TRPV6, a representative of the vanilloid subfamily of transient receptor potential (TRP) channels, is the principal calcium uptake channel that captures diet-delivered calcium ions in the gut4–6. TRPV6 is a constitutively open channel. TRPV6 is assembled of four subunits and contains a transmembrane domain (TMD) with the central ion channel pore and an intracellular skirt that is mostly built of ankyrin repeat domains connected to each other by three-stranded β-sheets, N-terminal helices, and C-terminal hooks. The TMD is composed of six transmembrane helices S1–S6 and a re-entrant pore loop (P-loop) between S5 and S6.

Cryo-EM micrographs for hTRPV6-CtD reconstituted in cNW30 nanodiscs in the presence of 114 µM THCV showed evenly dispersed particles with diverse angular coverage. The three-dimensional reconstruction of TRPV6THCV with four-fold rotational symmetry (C4) resulted in a cryo-EM map with the overall resolution of 2.79 Å. High-quality reconstruction of TRPV6THCV identifies three such densities per subunit as representing cholesteryl hemisuccinate (CHS), which was added during protein purification. The first one of the two corresponding THCV binding sites is formed by S5 and S6 of one subunit and S6 of the neighboring subunit and located in the portal connecting the pore and the membrane surrounding TMD. The second site is located next to the first one but it is more peripheral with respect to the pore, surrounded by lipids, including CHS molecules at the vanilloid site (at the interface of S5 and S6 of one subunit and S4 of the neighboring subunit) and at the interface of P-loop of one subunit and S6 of the neighboring subunit. Correspondingly, site 2 is unlikely to cause strong conformational changes in the protein and we propose that site 1 is the main inhibitory site of THCV. In contrast to the apo-state structures of hTRPV6, which have an open conducting pore, the pore in TRPV6THCV is in a fully closed conformation, hydrophobically sealed by the side chains of residues L574 and M578. According to the MD data, the only specific interaction that can stabilize the forward orientation of THCV is the hydrogen bond between the hydroxyl group of THCV and the carbonyl oxygen of L490. The rotation introduces a π-to-α transition in S6, making it entirely α-helical, causes a ~2 helical-turn shortening of S6, a ~2 helical-turn elongation of the TRP helix and repositions M578 so that its side chain points towards the channel pore center. In this position, M578 side chains hydrophobically seal the pore for water and ion conductance, finalizing the open-to-closed state transition. THCV therefore acts as a cog that inserts itself in a cogwheel mechanism of TRPV6 channel and ensures its transition from the open to closed state.

>[4x]MGLSLPKEKGLILCLWSKFCRWFQRRESWAQSRDEQNLLQQKRIWESPLLLAAKDNDVQALNKLLKYEDCKVHQRGAMGETALHIAALYDNLEAAMVLMEAAPELVFEPMTSELYEGQTALHIAVVNQNMNLVRALLARRASVSARATGTAFRRSPCNLIYFGEHPLSFAACVNSEEIVRLLIEHGADIRAQDSLGNTVLHILILQPNKTFACQMYNLLLSYDRHGDHLQPLDLVPNHQGLTPFKLAGVEGNTVMFQHLMQKRKHTQWTYGPLTSTLYDLTEIDSSGDEQSLLELIITTKKREARQILDQTPVKELVSLKWKRYGRPYFCMLGAIYLLYIICFTMCCIYRPLKPRTNNRTSPRDNTLLQQKLLQEAYMTPKDDIRLVGELVTVIGAIIILLVEVPDIFRMGVTRFFGQTILGGPFHVLIITYAFMVLVTMVMRLISASGEVVPMSFALVLGWCNVMYFARGFQMLGPFTIMIQKMIFGDLMRFCWLMAVVILGFASAFYIIFQTEDPEELGHFYDYPMALFSTFELFLTIIDGPANYNVDLPFMYSITYAAFAIIATLLMLNLLIAMMGDTHWRVAHERDELWRAQIVATTVMLERKLPRCLWPRSGICGREYGLGDRWFLRVEDRQDLNRQRIQRYAQAFHTRGSEDLDKDSVEK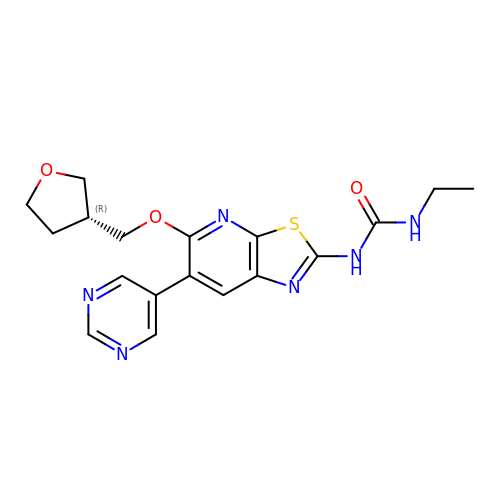1-ethyl-3-{6-(pyrimidin-5-yl)-5-[(3R)-tetrahydrofuran-3-ylmethoxy][1,3]thiazolo[5,4-b]pyridin-2-yl}urea | C18 H20 N6 O3 S | GVEJQEIIQCQRCC-LLVKDONJSA-N> CHGVSG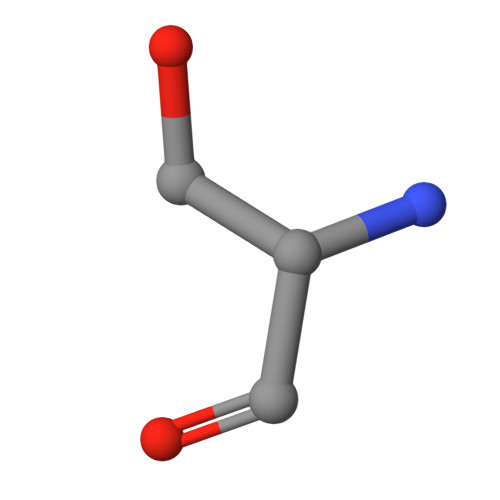SC>XGEIAQAL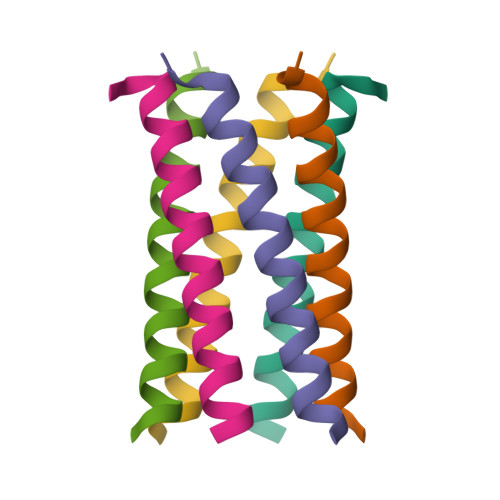KEIAKALKECAWALKEIAQALKGX[3x]Membrane bound histidine kinases (HKs) are ubiquitous sensors of extracellular stimuli in bacteria. Here, we used solid-state NMR in conjunction with crystallography, solution NMR and distance measurements to investigate the transmembrane signaling mechanism of a paradigmatic citrate sensing membrane embedded HK, CitA. In accordance with the naming of the PASc domain, the periplasmic domain is termed PASp here. The PASp and PASc domains are connected to the TM2 helix by two linkers: the PASp/TM2-linker and the TM2/PASc-linker (topology and domain organization shown in Fig. 1A).

Crystal structures of PASc reveal both anti-parallel and parallel dimer conformations. The N288D mutation in the PASc domain retains the same function as the wild-type (WT) CitA. When the function of the N288D CitA mutant was assessed by a β-galactosidase assay performed in E. coli CitA reporter strains, we found that N288D CitA unlike N304D of DcuS was fully functional, i.e., activated by citrate. The parallel dimer arrangement was previously reported in VicK11 but the anti-parallel arrangement had not been reported. Both the WT PASc and N288D PASc eluted as a dimer from a size exclusion column (SEC) down to a concentration of 1 μM, maintaining the dimer state in solution as hypothesized for membrane bound CitA. In agreement, the parallel or anti-parallel dimer arrangements were found to be the dominant forms in solution, respectively, for the WT or N288D PASc domain based on the following two methods. An inter-N308C distance of 41.3 Å was obtained in the N288D mutant PASc, which agrees with the expected distance in the anti-parallel dimer arrangement. While some populations of dimers at smaller separations in Fig. 2D cannot be excluded, the distribution of large distances about 41.3 Å indicates that the antiparallel arrangement dominates. For the PASc domain in CitA, this CEST effect was observed mainly in the residues from the N-terminal helices that form the dimer interface in both the anti-parallel and parallel arrangements. This indicates a dimer interface rearrangement of the PASc domain in isolation where the PASc domains switch most probably between the parallel and anti-parallel dimer forms, even when CEST does not reveal the identity of the conformations exchanging. Although this dimer exchange seen in the WT PASc is functionally more relevant, its occurrence in the N288D PASc mutant helps to rationalize why this point mutation does not disturb the functionality of the full length CitA.

>[2x]GSPEEIGLLYQEKQAILEAIREGIVAINQEGTITMVNQTALKLLGYDNERNVLGTPILQLIPHSRLPEVIRTGQAEYDDEMVLGGETVIADRIPIKNKQGRVIGAVSTFRNK Plasmoredoxin is a 22 ​kDa thiol–disulfide oxidoreductase involved in cellular redox regulatory processes and antioxidant defense. The structure reveals that plasmoredoxin, unique for malarial parasites, forms a new subgroup of thioredoxin-like proteins together with tryparedoxin, unique for kinetoplastids. The PfPlrx monomer (12–179 aa) contains a twisted seven-stranded, mixed β-sheet (β1, β2, β5, β4, β3, β6, β7), surrounded by five α-helices (α2 to α5). The longest helix (α2) in the PfPlrx structure comprises five turns with the typical thioredoxin active site motive WCXXC (W59, C60, K61, Y62, C63) at its N-terminal end.

We have obtained monoclinic (space group P21) and hexagonal crystals (space group P61) of PfPlrx from P. falciparum, both diffracted to 1.6 ​Å. The asymmetric unit of the monoclinic and hexagonal crystal types contained four and one monomers of PfPlrx, respectively. Manually rebuilding and subsequent refinement resulted in a PfPlrx model, comprising residues 12 to 179. Accordingly, we used this model to obtain the hexagonal structure. The five independent PfPlrx structures determined in the monoclinic (four monomers) and hexagonal (one monomer) crystal form are essentially similar. Superimposition of the monoclinic structures reveals an rmsd between 0.5 and 0.7 ​Å with about 160 residues, and comparison with the hexagonal structure shows an rmsd of 0.9 ​Å with 153 residues. All structures are in the reduced form, with an equal distance (3.8 ​Å) between the Sγ-atoms of the active site cysteines (C60, C63). The number of N-terminal residues seen in the electron density varies among the five structures. Furthermore, the N-terminal helix α1 is missing in the hexagonal structure. The asymmetric unit of the hexagonal crystal form contains one monomer, thus the dimer AA′ is formed by crystal contacts.

> MACQVDNPPKTYPNDKTAEYEKYANYMNYLYYYQNNELKKIDSSYFKDKYLGLFFGASWCKYCVTFIDSLNIFKKNFPNVEIIYIPFDRTYQEYQSFLKNTNFYALPFDNYLYICKKYQIKNLPSFMLITPNNNILVKDAAQLIKTDEYINNLKSLIKNYIIHPKTFQFNNRFFDLFRN>[2x]MGGYF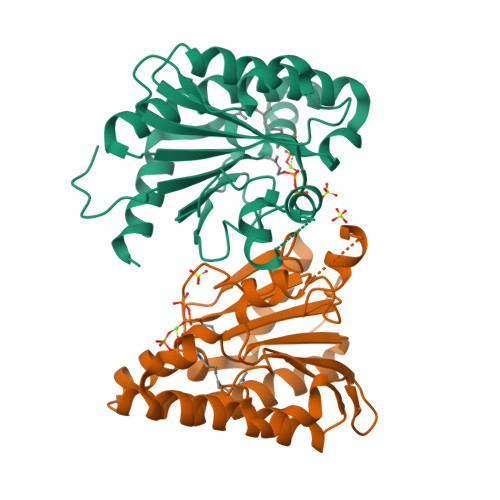LDTPKFKRLPGHIAIIPDGNRRWALDRGLEKHEGYKHGIVPGLELYDICVKIGIGEVTFFGFTQDNTKRPQIQRKAFVDACIKSVKELSKHDAELLVVGNTNSDMFPKELLAYTKRTKFGKGKVRINFLVNYGWYWDLTYAFENSSDSKKMIENIASAEIPRIDLLIRWGGRRRLSGMLPVQTVYSDIYVVDEMWPDFKPEHLFNALEFYQDQDITLGG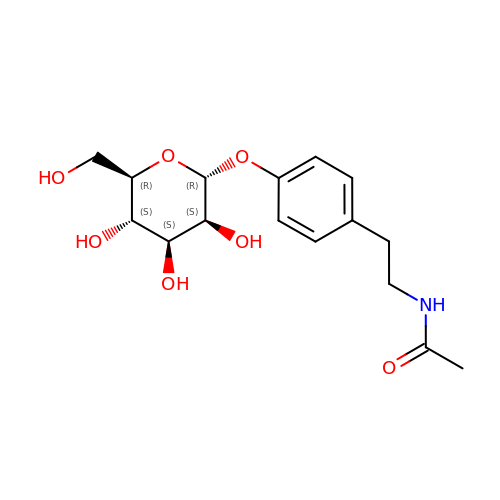~{N}-[2-[4-[(2~{R},3~{S},4~{S},5~{S},6~{R})-6-(hydroxymethyl)-3,4,5-tris(oxidanyl)oxan-2-yl]oxyphenyl]ethyl]ethanamide | C16 H23 N O7 | JVYCDFJBIOIPDL-OWYFMNJBSA-N>[2x]MNGNDPDIAGFKQQLVQMTAMRESQPPSIEIERQMFDAQHGAVPPAEGCLIEPISTGGVRGERITPKSADTSKALIYFHGGGHLFGSALSHRHLVSRLAAAAGVVAYNMEYRLAPENPYPAGLDDAEQAYRFVLAQGFKPEDIIVAGESAGGNLAAALLLKLRDQDLPQPAGAYLLSPWLDMSQSGASYEARGPHDPMITHNALTGCSAAYRAGASAEDPLISPAKADLADLPSLFIQVGADEVLLSDSVEFTRRAALAGLDVRLHVWANMVHAWPLFHFALPVSGLAAIDEAGAWISRQLGGHLEHHHHHH

In this work, we performed structural and biochemical characterization of the PMGL3 esterase, a novel member of the GDSAG motif subfamily of the bHSL family. The protein was obtained from the metagenomic DNA library constructed from the permafrost-derived microcosm. The PMGL3 esterase demonstrated low thermal stability with rapid inactivation upon incubation at 40 °C, which is typical for the cold-active enzymes. The PMGL3 demonstrated a typical fold for the bHSL family with however a unique tetrameric architecture.

PMGL3 subunit has a typical α/β bacterial HSL-like fold, consisting of two canonical domains—a CAP-domain and a catalytic domain. The CAP domain (residues 1–42) contains two α-helices (α1 and α2), while the large catalytic domain contains 8 β-strands (parallel β1 and β3-β8 as well as antiparallel to them β2) surrounded by 9 alpha-helices (α3-α11). Two PMGL3 subunits within an asymmetric unit form a homodimer, which is consistent with the current and previous SEC data. The dimeric interface is stabilized by 10 hydrogen bonds, 4 salt bridges as well as by hydrophobic interactions, thus involving α6, α9, α11 and β8 from each subunit and not affecting their CAP-domains. Further contact analysis revealed two possible tetrameric forms (T1 and T2) of PMGL3 within a crystal. T1 tetramer can be regarded as a dimer of dimers from the asymmetric unit and, thus, has two types of intermolecular interfaces–the dimeric interface, described above, and interdimeric interface. Analysis of tetramerization interfaces demonstrated that T1 has significantly greater buried area, number of polar interactions and free energy of assembly dissociation than T2. This indicates that T1 form is more stable and presumably the one found in solution, while T2 form is a result of crystal packing. PMGL3 tetramer has four active sites each made by the residues which belong to one subunit and are buried into the protein molecule. The oval entrance of about 13 × 7 Å is partly covered from the protein surface by the CAP-domain, allowing, however, access for the substrate through two large holes formed by a “bag handle”-like arc being composed of α1, α2 and the loop connecting these helices.>[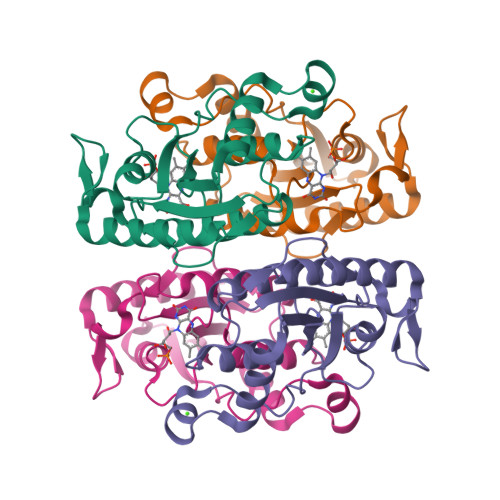2x]MAEKLQVVTLLGSLRKGSFNGMVARTLPKIAPASMEVNALPSIADIPLYDADVQQEEGFPATVEALAEQIRQADGVVIVTPEYNYSVPGGLKNAIDWLSRLPDQPLAGKPVLIQTSSMGVIGGARCQYHLRQILVFLDAMVMNKPEFMGGVIQNKVDPQTGEVIDQGTLDHLTGQLTAFGEFIQRVKILEGSS> MEFFGESWKKHLSGEFGKPYFIKLMGFVAEERKHYTVYPPPHQVF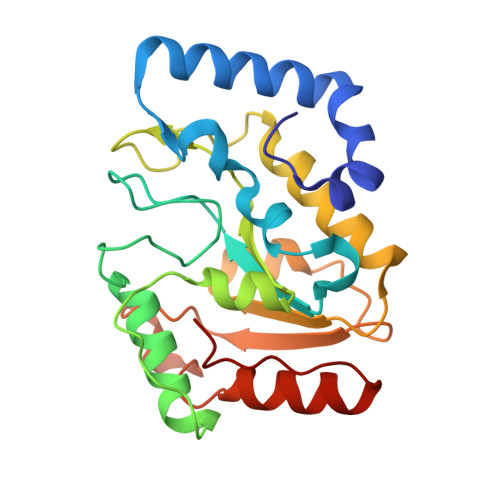TWTQMCDIKDVKVVILGQDPYHGPNQAHGLCFSVQRPVPPPPSLVNIYKELSTDIEDFVHPGHGDLSGWAKQGVLLLNAVLTVRAHQANSHKERGWEQFTDAVVSWLNQNSNGLVFLLWGSYAQKKGSAIDRKRHHVLQTAHPSPLSVYRGFFGCRHFSKTNELLQKSGKKPIDWKEL Berberine | C28 H27 N2 O4 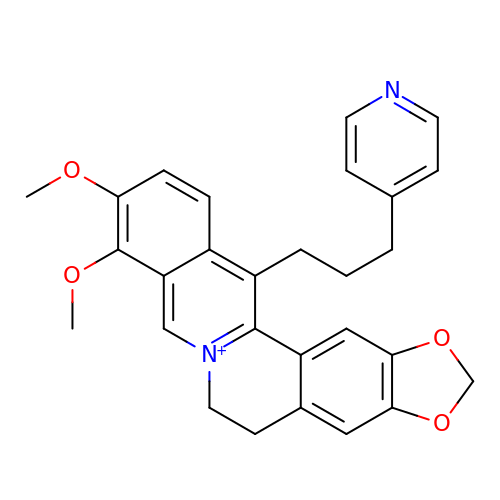| QVKHJFYKHMGTFF-UHFFFAOYSA-N> GSLKIAPANADFAFRFYYLIASETPGKNIFFSPLSISAAYAMLSLGACSHSRSQILEGLGFNLTELSESDVHRGFQHLLHTLNLPGHGLETRVGSALFLSHNLKFLAKFLNDTMAVYEAKLFHTNFYDTVGTIQLINDHVKKETRGKIVDLVSELKKDVLMVLVNYIYFKALWEKPFISSRTTPKDFYVDENTTVRVPMMLQDQEHHWYLHDRYLPCSVLRMDYKGDATVFFILPNQGKMREIEEVLTPEMLMRWNNLLRKRNFYKKLELHLPKFSISGSYVLDQILPRLGFTDLFSKWADLSGITKQQKLEAS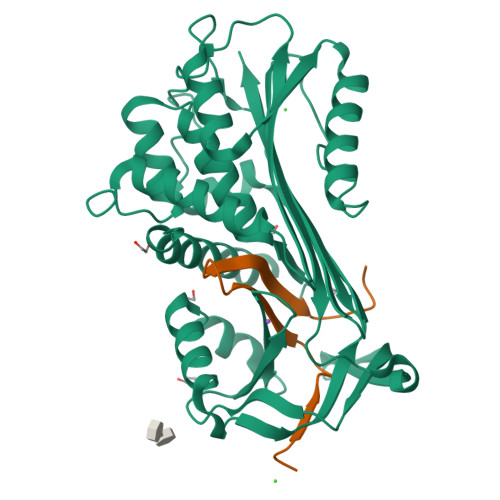KSFHKATLDVDEAGTEAAAATSFAIKF;> FSAQTNRHILRFNRPFLVVIFSTSTQSVLFLGKVVDPTKP> ASAKLPGDFGPPRGEPIHAVLTSPPLVPPPVNRTYPAKVIVELEVVEKEMQISEGVSYTFWTFGGTVPGSFIRVRQGDTVEFHLKNHPSSKMPHNIDLHGVTGPGGGAASSFTAPGHESQFTFKALNEGIYVYHCATAPVGMHIANGM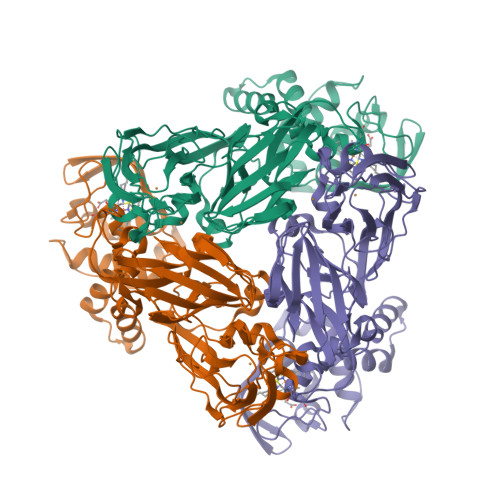YGLILVEPPEGLPKVDHEYYVMQGDFYTAGKYREKGLQPFDMEKAIDERPSYVLFNGAEGALTGDKALHAKVGETVRIFVGNGGPNLVSSFHVIGAIFDQVRYEGGTNVQKNVNTTLIPAGGAAVVKFTARVPGSYVLVDHSIFRAFNKGAMAILKIDGAENKLVYSGKELDSVYLGDRAAPNMSAVTKATQASVSGTLTVQDQVQAGRALFAGTCSVCHQGNGAGLPGVFPPLAKSDFLAADPKRAMNIVLHGLNGKIKVNGQEYDSVMPPMTQLNDDEVANILTYVLNSWDNPGGRVSAEDVKKVRAQPAPAKAVAEH> MSEPRFVHLRVHSDYSMIDGLAKTAPLVKKAAALGMPALAITDFTNLCGLVKFYGAGHGAGIKPIVGADFNVQCDLLGDELTHLTVLAANNTGYQNLTLLISKAYQRGYGAAGPIIDRDWLIELNEGLILLSGGRMGDVGRSLLRGNSALVDECVAFYEEHFPDRYFLELIRTGRPDEESYLHAAVELAEARGLPVVATNDVRFIDSSDFDAHEIRVAIHDGFTLDDPKRPRNYSPQQYMRSEEEMCELFADIPEALANTVEIAKRCNVTVRLGEYFLPQFPTGDMSTEDYLVKRAKEGLEERLAFLFPDEEERLKRRPEYDERLETELQVINQMGFPGYFLIVMEFIQWSKDNGVPVGPGRGSGAGSLVAYALKITDLDPLEFDLLFERFLNPERVSMPDFDVDFCMEKRDQVIEHVADMYGRDAVSQIITFGTMAAKAVIRDVGRVLGHPYGFVDRISKLIPPDPGMTLAKAFEAEPQLPEIYEADEEVKALIDMARKLEGVTRNAGKHAGGVVIAPTKITDFAPLYCDEEGKHPVTQFDKSDVEYAGLVKFDFLGLRTLTIINWALEMINKRRAKNGEPPLDIAAIPLDDKKSFDMLQRSETTAVFQLESRGMKDLIKRLQPDCFEDMIALVALFRPGPLQSGMVDNFIDRKHGREEISYPDVQWQHESLKPVLEPTYGIILYQEQVMQIAQVLSGYTLGGADMLRRAMGKKKPEEMAKQRSVFAEGAEKNGINAELAMKIFDLVEKFAGYGFNKSHSAAYALVSYQTLWLKAHYPAEFMAAVMTADMDNTEKVVGLVDECWRMGLKILPPDINSGLYHFHVNDDGEIVYGIGAIKGVGEGPIEAIIEARNKGGYFRELFDLCARTDTKKLNRRVLEKLIMSGAFDRLGPHRAALMNSLGDALKAADQ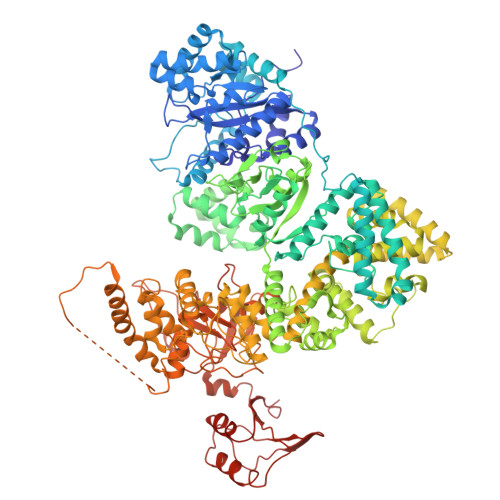HAKAEAIGQLDLFGVLAEEPEQIEQSYASCQPWPEQVVLDGERETLGLYLTGHPINQYLKEIERYVGGVRLKDMHPTERGKVITAAGLVVAARVMVTKRGNRIGICTLDDRSGRLEVMLFTDALDKYQQLLEKDRILIVSGQVSFDDFSGGLKMTAREVMDIDEAREKYARGLAISLTDRQIDDQLLNRLRQSLEPHRSGTIPVHLYYQRADARARLRFGATWRVSPSDRLLNDLRGLIGSEQVELEFD UNDECYL-PHOSPHINIC ACID BUTYL ESTER | C15 H33 O2 P | 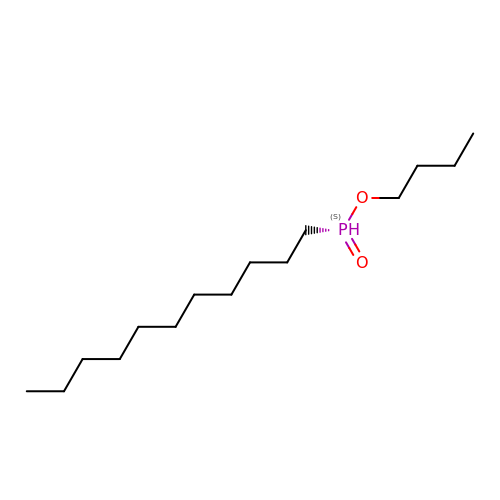QCBLJDSWVGAXQB-UHFFFAOYSA-N> GPVCAEASDVYSPCMIASTPPAPFSDVTAVTFDLINGKITPVGDDNWNTHIYNPPIMNVLRTAAWKSGTIHVQLNVRGAGVKRADWDGQVFVYLRQSMNPESYDARTFVISQPGSAMLNFSFDIIGPNSGFEFAESPWANQTTWYLECVATNPRQIQQFEVNMRFDPNFRVAGNILMPPFPLSTETPPL;> MEQNLFALSLDDTSSVRGSLLDTKFAQTRVLLSKAMAGGDVLLDEYLYDVVNGQDFRATVAFLRTHVITGKIKVTATTNISDNSGCCLMLAINSGVRGKYSTDVYTICSQDSMTWNPGCKKNFSFTFNPNPCGDSWSAEMISRSRVRMTVICVSGWTLSPTTDVIAKLDWSIVNEKCEPTIYHLADCQNWLPLNRWM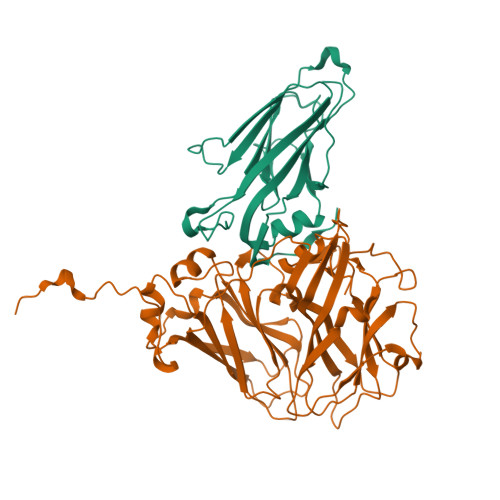GKLTFPQGVTSEVRRMPLSIGGGAGATQAFLANMPNSWISMWRYFRGELHFEVTKMSSPYIKATVTFLIAFGNLSDAFGFYESFPHRIVQFAEVEEKCTLVFSQQEFVTAWSTQVNPRTTLEADGCPYLYAIIHDSTTGTISGDFNLGVKLVGIKDFCGIGSNPGIDGSRLL>[2x]TIQGSIVAIVTPMLKDGGVDWKSLEKLVEWHIEQGTNSIVAVGTTGEASTLSMEEHTQVIKEIIRVANKRIPIIAGTGANSTREAIELTKAAKDLGADAALLVTPYYNKPTQEGLYQHY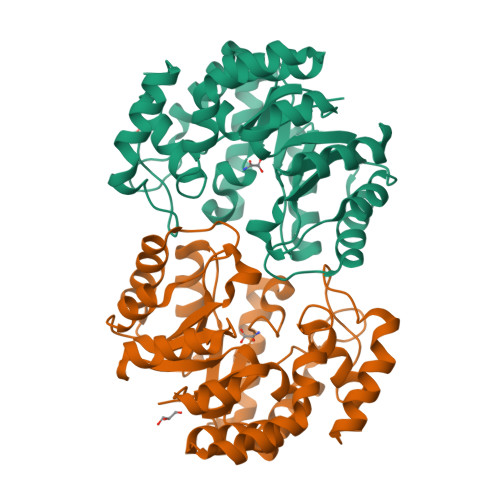KAIAEAVELPLILYNVPGRTGVDLSNDTAVRLAEIPNIVGIKDATGDVPRGKALIDALNGKMAVYSGDDETAWELMLLGADGNISVTANIAPKAMSEVCAVAIAKDEQQAKTLNNKIANLHNILFCESNPIPVKWALHEMGLIDTGIRLPLTPLAEQYREPLRNALKDAGII> SMNGVLIPHTPIAVDFWSLRRAGTARLFFLSHMHSDHTVGLSSTWARPLYCSPITAHLLHRHLQVSKQWIQALEVGESHVLPLDEIGQETMTVTLLDANHCPGSVMFLFEGYFGTILYTGDFRYTPSMLKEPALTLGKQIHTLYLDNTNCNPALVLPSRQEAAHQIVQLIRKHPQHNIKIGLYSLGKESLLEQLALEFQTWVVLSPRRLELVQLLGLADVFTVEEKAGRIHAVDHMEICHSNMLRWNQTHPTIAILPTSRKIHSSHPDIHVIPYSDHSSYSELRAFVAAL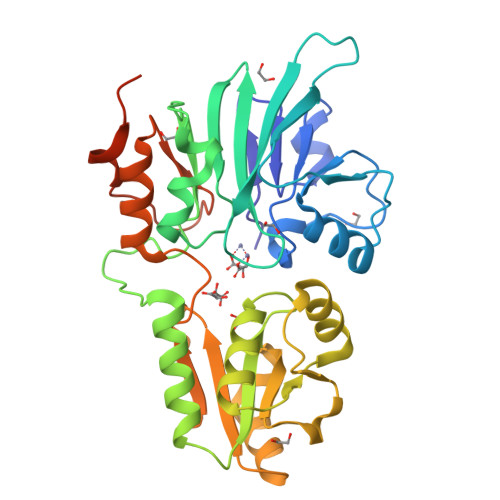KPCQVVPIVSRRPCGGFQDSLSPRISVPLIPDSVQQYMSSFSRKPS> MAHHHHHHVGTGSNDDDDKSPDPTQDVREPPALKYGIVLDAGSSHTSMFVYKWPADKENDTGIVGQHSSCDVQGGGISSYANDPSKAGQSLVRCLEQALRDVPRDRHASTPLYLGATAGMRLLNLTSPEATARVLEAVTQTLTQYPFDFRGARILSGQDEGVFGWVTANYLLENFIKYGWVGRWIRPRKGTLGAMDLGGASTQITFETTSPSEDPGNEVHLRLYGQHYRVYTHSFLCYGRDQILLRLLASALQIHRFHPCWPKGYSTQVLLQEVYQSPCTMGQRPRAFNGSAIVSLSGTSNATLCRDLVSRLFNISSCPFSQCSFNGVFQPPVAGNFIAFSAFYYTVDFLTTVMGLPVGTLKQLEEATEITCNQTWTELQARVPGQKTRLADYCAVAMFIHQLLSRGYHFDERSFREVVFQKKAADTAVGWALGYMLNLTNLIPADLPGLRKG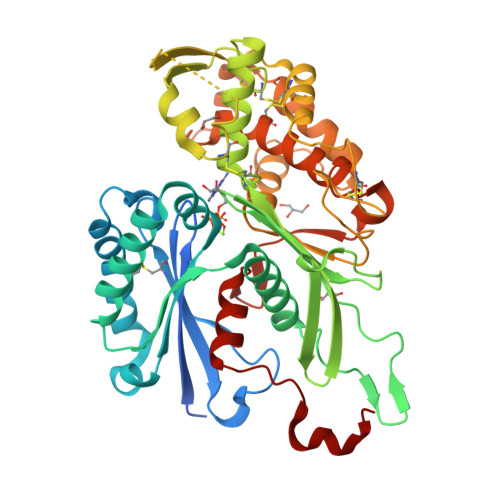THFS>[2x]MGGSHHHHHHGMASLAPGSSRVELFKRQSSKVPFEKDGKVTERVVHSFRLPALVNVDGVMVAIADARYETSFDNSLIDTVAKYSVDDGE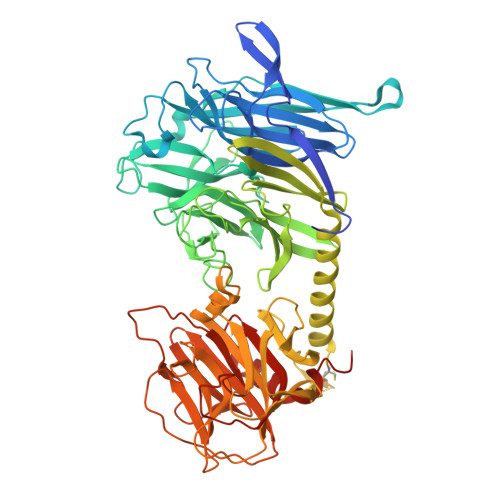TWETQIAIKNSRASSVSRVVDPTVIVKGNKLYVLVGSYNSSRSYWTSHGDARDWDILLAVGEVTKSTAGGKITASIKWGSPVSLKEFFPAEMEGMHTNQFLGGAGVAIVASNGNLVYPVQVTNKKKQVFSKIFYSEDEGKTWKFGKGRSAFGCSEPVALEWEGKLIINTRVDYRRRLVYESSDMGNTWLEAVGTLSRVWGPSPKSNQPGSQSSFTAVTIEGMRVMLFTHPLNFKGRWLRDRLNLWLTDNQRIYNVGQVSIGDENSAYSSVLYKDDKLYCLHEINSNEVYSLVFARLVGELRIIKSVLQSWKNWDSHLSSICTPADPAASSSERGCGPAVTTVGLVGFLSHSATKTEWEDAYRCVNASTANAERVPNGLKFAGVGGGALWPVSQQGQNQRYHFANHAFTLVASVTIHEVPKGASPLLGASLDSSGGKKLLGLSYDKRHQWQPIYGSTPVTPTGSWEMGKRYHVVLTMANKIGSVYIDGEPLEGSGQTVVPDERTPDISHFYVGGYKRSGMPTDSRVTVNNVLLYNRQLNAEEIRTLFLSQDLIGTEAHMD>[12x]EMSCAEKLLKVLSFGLWNPTYSRSERQSFQELLTVLEPVYPLPNELGRVSARFSDGSSLRISVTNSE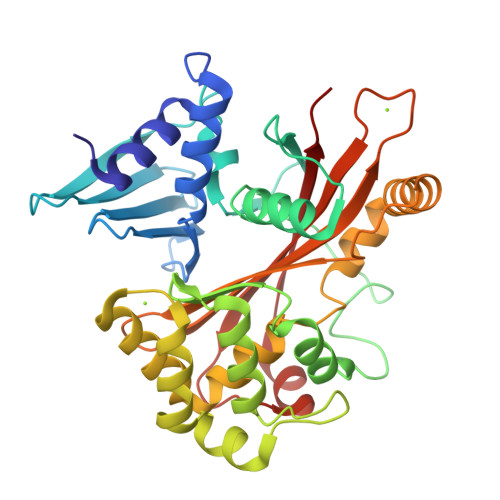SIEAEIRTPDNEKITVLLESNEQNRLLQSLPIDRHMPYIQVHRALSEMDLTDTTSMRNLLGFTSKLSTTLIPHNAQTDPLSGPTPFSSIFMDTCRGLGNAKLSLNGVDIPANAQMLLRDALGLKDTHSSPSRNVIDHGISRHDAEQIARESSGSDNQKAEVVEFLCHPEAATAICSAFYQSFNVPALTLTHERISKASEYNAERSLDTPNACINISISQSSDGNIYVTSHTGVLIMAPEDRPNEMGMLTNRTSYEVPQGVKCTIDEMVRALQPRYAASETYLQN>SNATNTDTNSTNNSPNNTTNTTTNVTTTSDKNTIPIGIALAQTSNVALLGQEQVAGAKIAEKYFNDKGGVNGTPIKLIFQDTAGDEAGTINAFQTLINKDKVVGIVGPTLSQQAFSANPIAERAKVPVVGPSNTAKGIPEIGDYVARVSAPVSVVAPNSVKAALKQNPNIKKVAVFFAQNDAFSKSETEIFQQTVKDQGLELVTVQKFQTTDTDFQSQATNAINLKPDLVIISGLAADGGNLVRQLRELGYQGAIIGGDGLNTSNVFAVCKALCDGVLIAQAYSPEYTGEINKAFRQAYVDQYKKEPPQFSAQAFAAVQVYV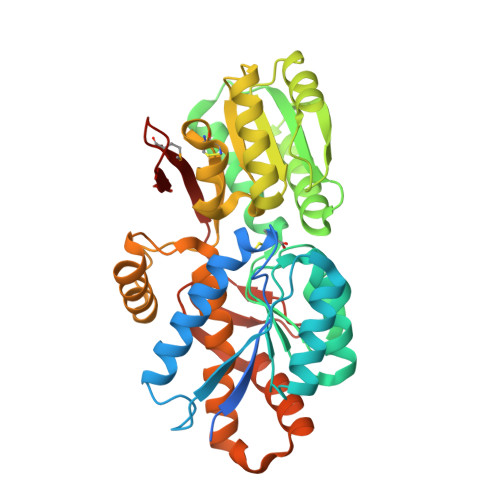ESLKALDTKNKVSKIQLPELRTELNKQLLTGKYNTPLGEISFTPIGEVVQKDFYVAQIKMEKDGSQGKFTFLK[2x]>[4x]MAFMKKYLLPILGLFMAYYYYSANEEFRPEMLQGKKVIVTGASKGIGREMAYHLAKMGAHVVVTARSKETLQKVVSHCLELGAASAHYIAGTMEDMTFAEQFVAQAGKLM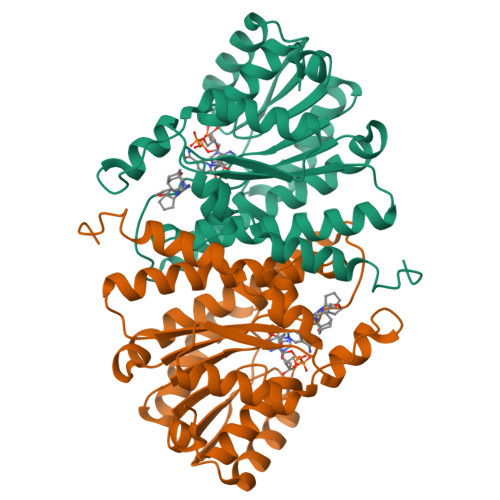GGLDMLILNHITNTSLNLFHDDIHHVRKSMEVNFLSYVVLTVAALPMLKQSNGSIVVVSSLAGKVAYPLVAAYSASKFALDGFFSSIRKEYSVSRVNVSITLCVLGLIDTETAMKAVSGIVHMQAAPKEECALEIIKGGALRQEEVYYDSSRWTTLLIRNPSRKILEELYSTSYNMDRFINK> MATSSMSKGCFVFKPNSKKRKISLPIEDYFNKGKNEPEDSKLRFETYQLIWQQMKSENERLQEELNKNLFDNLIEFLQKSHSGFQKNSRDL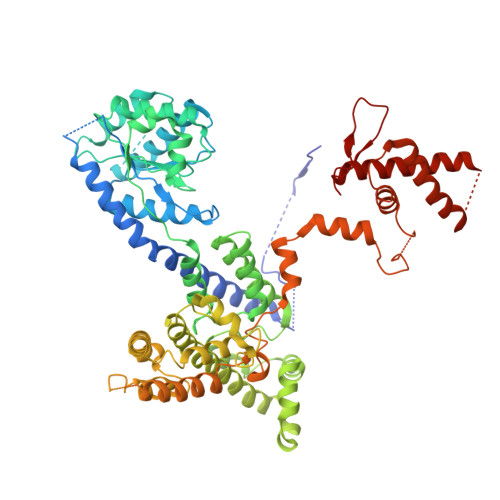GGQIKLREIPTAALVLGVNVTDHDLTFGSLTEALQNNVTPYVVSLQAKDCPDMKHFLQKLISQLMDCCVDIKSKEEESVHVTQRKTHYSMDSLSSWYMTVTQKTDPKMLSKKRTTSSQWQSPPVVVILKDMESFATKVLQDFIIISSQHLHEFPLILIFGIATSPIIIHRLLPHAVSSLLCIELFQSLSCKEHLTTVLDKLLLTTQFPFKINEKVLQVLTNIFLYHDFSVQNFIKGLQLSLLEHFYSQPLSVLCCNLPEAKRRINFLSNNQCENIRRLPSFRRYVEKQASEKQVALLTNERYLKEETQLLLENLHVYHMNYFLVLRCLHKFTSSLPKYPLGRQIRELYCTCLEKNIWDSEEYASVLQLLRMLAKDELMTILEKCFKVFKSYCENHLGSTAKRIEEFLAQFQSLDETKEEEDASGSQPKGLQKTDLYHLQKSLLEMKELRRSKKQTKFEVLRENVVNFIDCLVREYLLPPETQPLHEVVYFSAAHALREHLNAAPRIALHTALNNPYYYLKNEALKSEEGCIPNIAPDICIAYKLHLECSRLINLVDWSEAFATVVTAAEKMDANSATSEEMNEIIHARFIRAVSELELLGFIKPTKQKTDHVARLTWGGC> GSHMSAEVIHQVEEALDTDEKEMLLFLCRDVAIDVVPPNVRDLLDILRERGKLSVGDLAELLYRVRRFDLLKRILKMDRKAVETHLLRNPHLVSDYRVLMAEIGEDLDKSDVSSLIFLMKDYMGRGKIS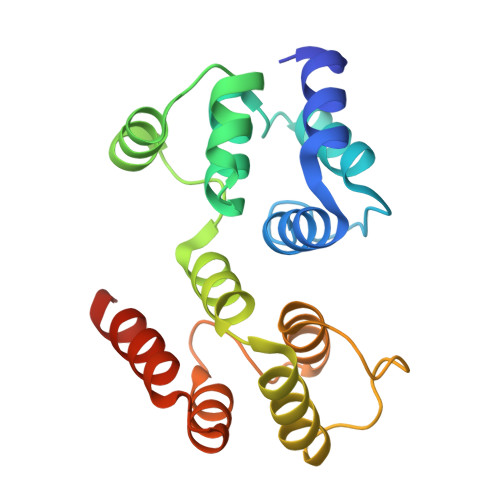KEKSFLDLVVELEKLNLVAPDQLDLLEKCLKNIHRIDLKTKIQKYKQSVQGAGTS>[8x]MPKPYVAINMVEVRNDPKTLELFGKVGPKVCMVTARHPGFVGFQNHVQIGVVPLGTRWGGAKMEMSQEMHSLMLMQYTFWKNWKDHEEMHKQNWANLFRLCLQCADQMIWGPYEPLYEIVYANMPLNTEMTDFTVMVGKKFAAGEAVSIPPISQPYGKRVVAFGEHIVKEGLENQFEEYAIKTLEAFRSAPGFLGGMILKEIGVSPLGSLQLNAKGFHQILETANGMDVPEPVTIYEAPEFRNRPQRYIVHTEWSDTNALMFGLGRVLIYPEVRQIHDKVLDTLVYGPYIRVLNPMMEGTYWREYLNEYHL

Sulfur oxygenase reductases (SORs) are present in thermophilic and mesophilic archaea and bacteria, and catalyze oxygen-dependent oxygenation and disproportionation of elemental sulfur. SOR has a hollow, spherical homo-24-mer structure and reactions take place at active sites inside the chamber. Here, we report the biochemical and structural characterizations of SORs from the thermoacidophilic archaeon Sulfurisphaera tokodaii (StSOR) and present high-resolution structures determined by X-ray crystallography and cryogenic electron microscopy (cryo-EM). Each monomer has an 8-stranded β barrel core surrounded by 10 α helices.

The crystal structure was determined at 1.73 Å resolution using a crystal belonging to the cubic I23 space group. The crystal contains 8 monomers per asymmetric unit and the 24-mer with a pseudo-432 point group was generated by applying the crystallographic 3-fold rotation axis. The final model contains residues from Pro2 to Leu311 of all chains without a disordered region. The iron atom in the active site is ligated to His86, His90, Glu114 (bidentate) and two waters designated as Wat1 and Wat2. The octahedral iron site in the StSOR crystal structure is similar to that of AaSOR while the iron site of AtSOR was five-coordinated with only one water (Wat2 as the opposite ligand to His86). StSOR also has the three conserved cysteines with distances to the iron atom of 9.5–13.0 Å, and Cys31 is located on the route from the central cavity of the chamber to the catalytic iron. Electron density maps around the Sγ atoms of the cysteine residues clearly indicate that all are mainly present as free thiols in the StSOR crystal. Phe133, Val137, and Phe141 are lined inside the chimney to form a hydrophobic channel that is suitable for S0 entry. The hydrophobic side chains of the chimneys were clearly observed in the electron density map of the crystal structure. Due to the crystal packing effect, the chimneys have relatively low B-factor values compared to the interior regions of the hollow sphere.> PLSILVRNERGHSNIYEVFLTQTVDTLKKKVSQREQV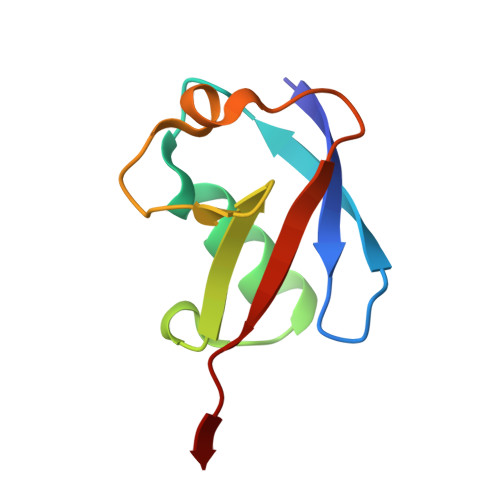HEDQFWLSFEGRPMEDKELLGEYGLKPQCTVIKHLRLRG>METSKEKTITSPGPYIVRLLNSSLNGCEFPLLTGRTLFVVGQSDALTASGQLPDIPADSFFIPLDHGGVNFEIQVDTDATEIILHELKEGNSESRSVQLNTPIQVGELLILIRPESEPWVPEQPEKLETSAKKNEPRFKNGIVAALAGFFILGIGTVGTLWILNSPQRQAAELDSLLGQ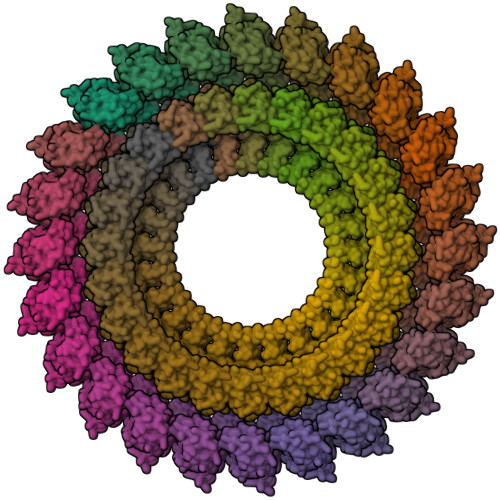EKERFQVLPGRDKMLYVAAQNERDTLWARQVLARGDYDKNARVINENEENKRISIWLDTYYPQLAYYRIHFDEPRKPVFWLSRQRNTMSKKELEVLSQKLRALMPYADSVNITLMDDVTAAGQAEAGLKQQALPYSRRNHKGGVTFVIQGALDDVEILRARQFVDSYYRTWGGRYVQFAIELKDDWLKGRSFQYGAEGYIKMSPGHWYFPSPL[24x];>[24x]MIRRYLYTFLLVMTLAGCKDKDLLKGLDQEQANEVIAVLQMHNIEANKIDSGKLGYSITVAEPDFTAAVYWIKTYQLPPRPRVEIAQMFPADSLVSSPRAEKARLYSAIEQRLEQSLQTMEGVLSARVHISYDIDAGENGRPPKPVHLSALAVYERGSPLAHQISDIKRFLKNSFADVDYDNISVVLSERSDAQLQAPGTPVKRNSFATSWIVLIILLSVMSAGFGVWYYKNHYARNKKGITADDKAKSSNE6-[(5-fluoro-4-methylpyridin-2-yl)amino]-4-[(2-methoxy-3-{[(pyridin-2-yl)methyl]carbamoyl}phenyl)amino]-N-methylpyridine-3-carboxamide 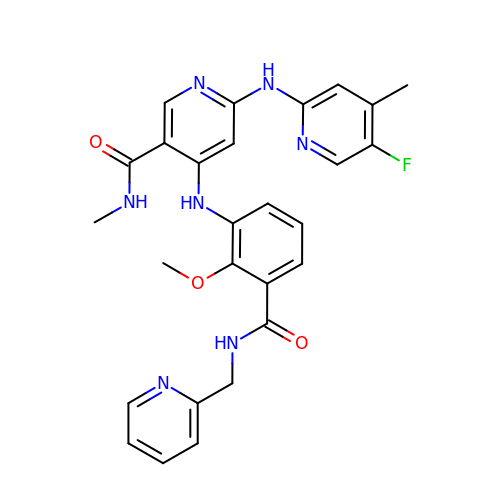| C27 H26 F N7 O3 | OXIRLLVPYPWPEK-UHFFFAOYSA-N(2R)-6-amino-2-[(2E)-2-({3-hydroxy-2-methyl-5-[(phosphonooxy)methyl]pyridin-4-yl}methylidene)hydrazin-1-yl]hexanoic 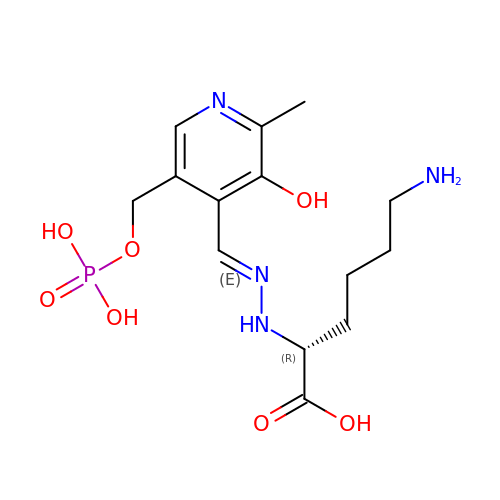acid | C14 H23 N4 O7 P | OUJFSRRLFCKCMC-UHFFFAOYSA-N>[2x]MFIINSDFHRGNMEQYQKAQKLSFDPAELLRTSLNVGDIVLLKQCTSELTMCVNLPQSTTDPRYTFAKKDGTLVYAMKNSVILRIPKDLPEEVNQLLKRESNHPYQKIGTIKNSSNETEILPVLTRQLIVSFTLATFTKFAWTQLPIVLKKLELIHRYLQDSRGSKHVN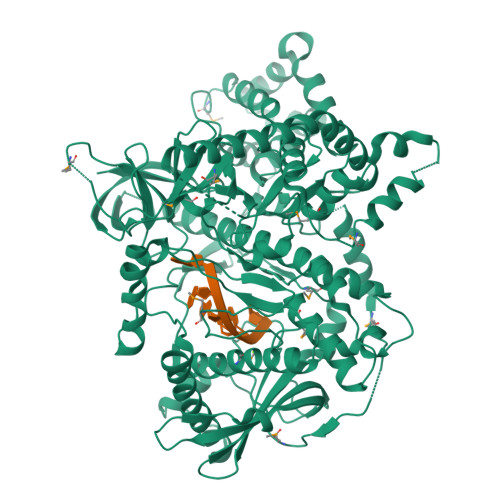FMSLVRIIKNLNIKEATDAINGDAYVRKVIDESMSVVNKSIDPTTLLATYWGVREQQQNNLWGSVYTNTALLSPTTVAVLPLKKAHLFYQEVITRLESNDYQEIKAFAKLVNDKDYHSIAKRYDYIRTLLNDYAAGNIEENAVLTTIISKIFRHIDMYRDQDVTRSLCGKLLVEISPQSNSSNFILGNWDLNIPKSSGISSVEQKLYDTAMPTIVSDTDRYDFGDMPVFCIDSEDAHEINDGISIEELDGVRSRIHIHIADPAGLFPESFDYTKSGISDDVLRVSLKRAFTTYLPDLVVPMLPKSFCNRADLGKHDRKTETISFSFELVNKEDGGLHVDYDTFQVRLGIVSNFPKVTYDKVDSILNGDDNSLPSKQKKQLELLHTLATKLLHKRIHDDNAVVFGDGFNKGLVSLSPDDDGELCIPTFYDQSQTKSTLLVSEFMILTNKLCAAFFQENKIPGVYRCYNGLNLGNQAKAQFELLKENIKLGKLPSLKDITKISSQLSSSFYSPFPLPHKMIGNTAYLTVTSPMRRGPDLINHLQLHRFLKKLPLCFKQEYLDQYVWSFQARADILKIFQRHSSTYWTLKHLEQSGTKTHDVIVTSVPQNGTVNCLFPEYSYARGTLKLDPAMKKIPRIGDTIRHCKVESIHPLDGILTLTHVNRK> GLGKGGA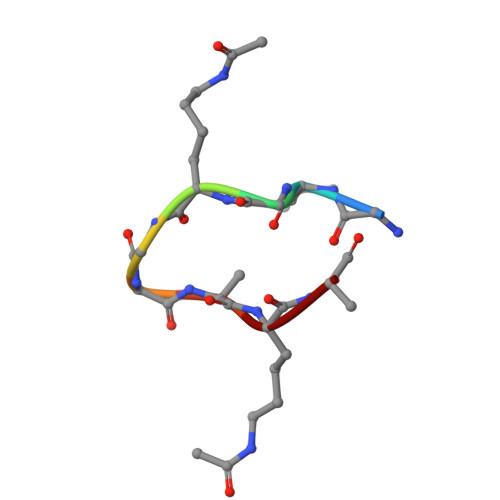KA5'-O-{[({[2-({[5-(DIMETHYLAMINO)NAPHTHALEN-1-YL]SULFONYL}AMINO)ETHYL]OXY}PHOSPHINATO)OXY]PHOSPHINATO}CYT 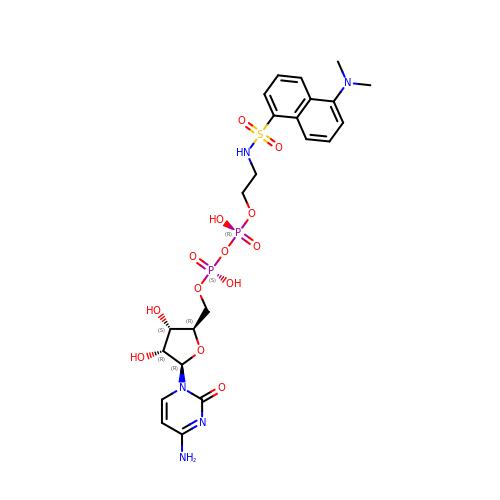| C23 H31 N5 O13 P2 S | OXPWLEWKRGQJQO-BRKWEVRTSA-N>CLAEGTRIFDPVTGTTHRIEDVVDGRKPIHVVAAAKDGTLHARPVVSWFDQGTRDVIGLRIAGGAILWATPDHKVLTEYGWRAAGELRKGDRVAQPRRFDGFGDSAPIPARVQALADALDDKFLH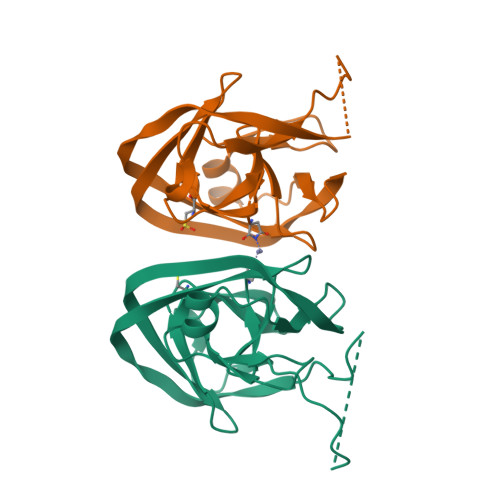DMLAEELRYSVIREVLPTRRARTFDLEVEELHTLVAEGVVVHN[2x]> MGSHHHHHHSQDPMMSRLKTAVYDYLNDVDI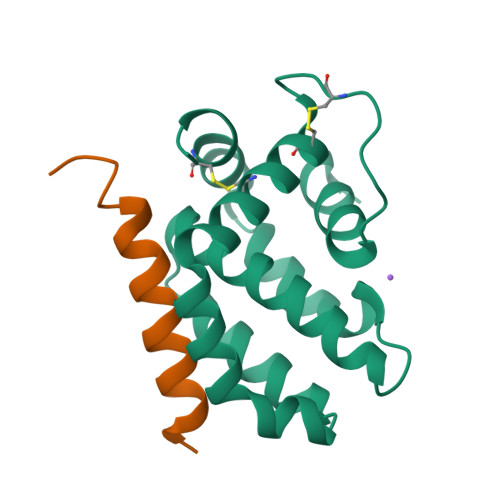TECTEMDLLCQLSNCCDFINETYAKNYDTLYDIMERDILSYNIVNIKNTLTFALRDASPSVKLATLTLLASVIKKLNKIQHTDAAMFSEVIDGIVAEEQQVIGFIQKKCKYNTT;> PSSTMGQVGRQLAIIGDDINRRYDSE>[2x]GPTPEAPYTEIEHLVQSVCKSYR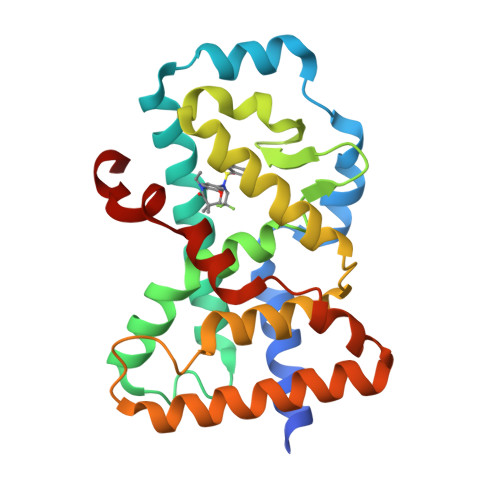ETCQLRLEDLLRQRSNIFSREEVTGYQRKSMWEMWERCAHHLTEAIQYVVEFAKRLSGFMELCQNDQIVLLKAGAMEVVLVRMCRAYNADNRTVFFEGKYGGMELFRALGCSELISSIFDFSHSLSALHFSEDEIALYTALVLINAHRPGLQEKRKVEQLQYNLELAFHHHLCKTHRQSILAKLPPKGKLRSLCSQHVERLQIFQ> MSKFLDRFRYFKQKGETFADGHGQLLNTNRDWEDGYRQRWQHDKIVRSTCGVNCTGSCSWKIYVKNGLVTWETQQTDYPRTRPDLPNHEPRGCPRGASYSWYLYSANRLKYPMMRKRLMKMWREAKALHSDPVEAWASII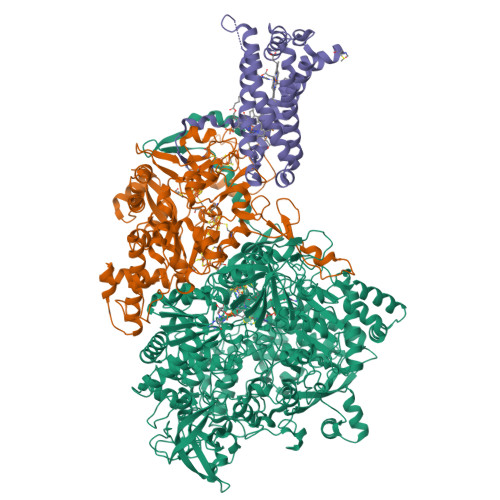EDADKAKSFKQARGRGGFVRSSWQEVNELIAASNVYTIKNYGPDRVAGFSPIPAMSMVSYASGARYLSLIGGTCLSFYDWYCDLPPASPQTWGEQTDVPESADWYNSSYIIAWGSNVPQTRTPDAHFFTEVRYKGTKTVAVTPDYAEIAKLCDLWLAPKQGTDAAMALAMGHVMLREFHLDNPSQYFTDYVRRYTDMPMLVMLEERDGYYAAGRMLRAADLVDALGQENNPEWKTVAFNTNGEMVAPNGSIGFRWGEKGKWNLEQRDGKTGEETELQLSLLGSQDEIAEVGFPYFGGDGTEHFNKVELENVLLHKLPVKRLQLADGSTALVTTVYDLTLANYGLERGLNDVNCATSYDDVKAYTPAWAEQITGVSRSQIIRIAREFADNADKTHGRSMIIVGAGLNHWYHLDMNYRGLINMLIFCGCVGQSGGGWAHYVGQEKLRPQTGWQPLAFALDWQRPARHMNSTSYFYNHSSQWRYETVTAEELLSPMADKSRYTGHLIDFNVRAERMGWLPSAPQLGTNPLTIAGEAEKAGMNPVDYTVKSLKEGSIRFAAEQPENGKNHPRNLFIWRSNLLGSSGKGHEFMLKYLLGTEHGIQGKDLGQQGGVKPEEVDWQDNGLEGKLDLVVTLDFRLSSTCLYSDIILPTATWYEKDDMNTSDMHPFIHPLSAAVDPAWEAKSDWEIYKAIAKKFSEVCVGHLGKETDIVTLPIQHDSAAELAQPLDVKDWKKGECDLIPGKTAPHIMVVERDYPATYERFTSIGPLMEKIGNGGKGIAWNTQSEMDLLRKLNYTKAEGPAKGQPMLNTAIDAAEMILTLAPETNGQVAVKAWAALSEFTGRDHTHLALNKEDEKIRFRDIQAQPRKIISSPTWSGLEDEHVSYNAGYTNVHELIPWRTLSGRQQLYQDHQWMRDFGESLLVYRPPIDTRSVKEVIGQKSNGNQEKALNFLTPHQKWGIHSTYSDNLLMLTLGRGGPVVWLSEADAKDLGIADNDWIEVFNSNGALTARAVVSQRVPAGMTMMYHAQERIVNLPGSEITQQRGGIHNSVTRITPKPTHMIGGYAHLAYGFNYYGTVGSNRDEFVVVRKMKNIDWLDGEGNDQVQESVK;> MKIRSQVGMVLNLDKCIGCHTCSVTCKNVWTSREGVEYAWFNNVETKPGQGFPTDWENQEKYKGGWIRKINGKLQPRMGNRAMLLGKIFANPHLPGIDDYYEPFDFDYQNLHTAPEGSKSQPIARPRSLITGERMAKIEKGPNWEDDLGGEFDKLAKDKNFDNIQKAMYSQFENTFMMYLPRLCEHCLNPACVATCPSGAIYKREEDGIVLIDQDKCRGWRMCITGCPYKKIYFNWKSGKSEKCIFCYPRIEAGQPTVCSETCVGRIRYLGVLLYDADAIERAASTENEKDLYQRQLDVFLDPNDPKVIEQAIKDGIPLSVIEAAQQSPVYKMAMEWKLALPLHPEYRTLPMVWYVPPLSPIQSAADAGELGSNGILPDVESLRIPVQYLANLLTAGDTKPVLRALKRMLAMRHYKRAETVDGKVDTRALEEVGLTEAQAQEMYRYLAIANYEDRFVVPSSHRELAREAFPEKNGCGFTFGDGCHGSDTKFNLFNSRRIDAIDVTSKTEPHP;> MQFLNMFFFDIYPYIAGAVFLIGSWLRYDYGQYTWRAASSQMLDRKGMNLASNLFHIGILGIFVGHFFGMLTPHWMYEAWLPIEVKQKMAMFAGGASGVLCLIGGVLLLKRRLFSPRVRATTTGADILILSLLVIQCALGLLTIPFSAQHMDGSEMMKLVGWAQSVVTFHGGASQHLDGVAFIFRLHLVLGMTLFLLFPFSRLIHIWSVPVEYLTRKYQLVRARH>MAVPFVEDWDLVQTLGEGAYGEVQLAVNRVTEEAVAVKIVDMKRAVDCPENIKKEICILKMLNHENVIKFYGHRREGNIQYLFMELASGG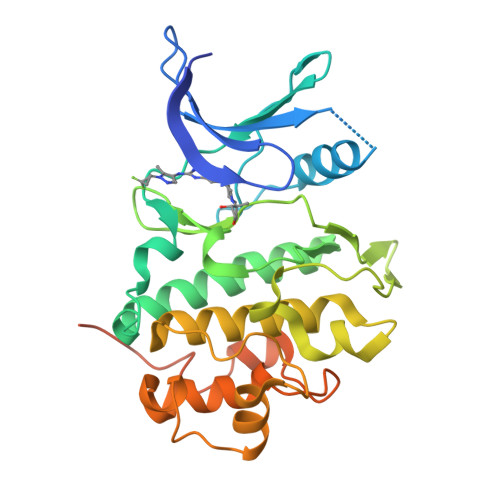SLFDRIEPDIGMPEPDAQRFFHQLMAGVVYLHGIGITHRDIKPHNLLLDERDNLKIADYSLATVFRYNNRERLLNKMCGTLPYVAPELLKRREFHAEPVDVWSCGIVLTAMLAGELPWDQPSDSCQEYSDWKEKKTYLNPWKKIDSAPLALLHKILVENPSARITIPDIKKDRWYNKPLKKGAKRPRVTSGGVSESPSGHHHHHHHH[2x]>GPHMSDHKFLTQAVEEAYKGVDCGDGGPFGAVIVHNNEVVASCHNMVLKYTDPTAHAEVTAI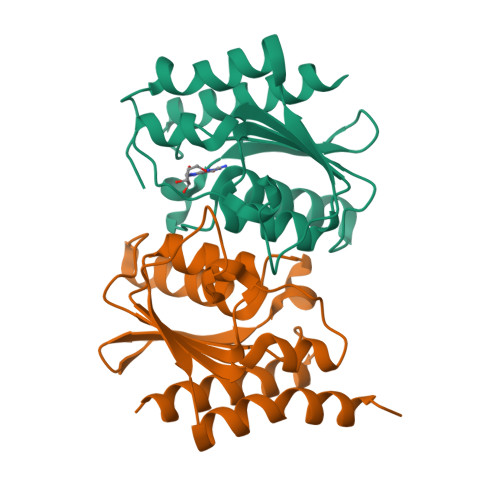REACKKLNKIELSECEIYASCEPCPMCFGAIHLSRLKRLVYGAKAEAAIAIGFDDFIADALRGTGVYQKSSLEIKKADGNGAAIAEQVFQNTKEKFRLF[2x]>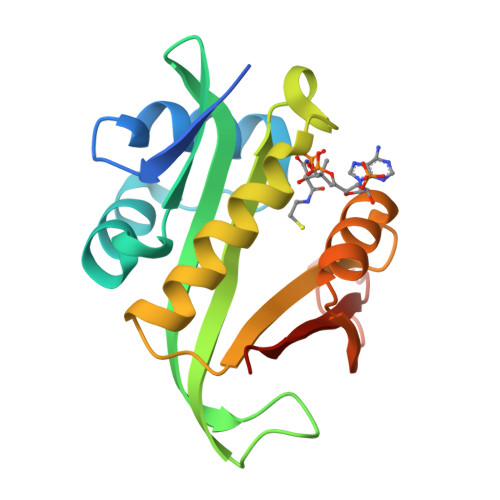[2x]MELAEKDKGRDFTLRNARMDDIDQIIKINRLTLPENYPYYFFVEHLKEYGLAFFVAIVDNSVVGYIMPRIEWGFSNIKQLPSLVRKGHVVSIAVLEEYRRKGIATTLLEASMKSMKNDYNAEEIYLEVRVSNYPAIALYEKLNFKKVKVLKGYYADGEDAYLMARPLHHHHHH> MALDKSIVVNLTSRL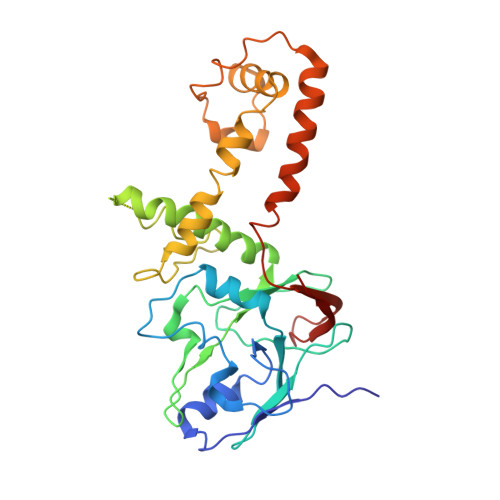FADELAALQSKIGSVLPLGDCHRLQNIQALGLGCVCSRETSPDYIQIMQYLSKCTLAVLEEVRPDSLRLTRMDPSDNLQIKNVYAPFFQWDSNTQLAVLPPLFSRKDSTIVLESNGFDIVFPMVVPQQLGHAILQQLLVYHIYSKISAGAPGDVNMAELDLYTTNVSFMGRTYRLDVDNTDPRTALRVLDDLSMYLCILSALVPRGCLRLLTALVRHDRHPLTEVFEGVVPDEVTRIDLDQLSVPDDITRMRVMFSYLQSLSSIFNLGPRLHVYAYSAETLAASCWYSPR> GCGCAGCCTGTACGGACATCA;> CCGTACA;> GGCTGC;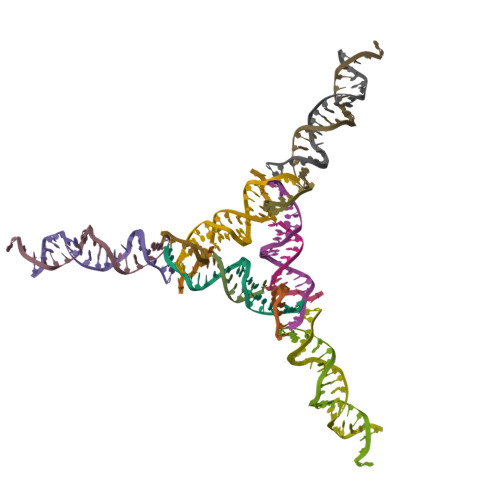> TCTGATGT;> GATGCTGACGTAGTAGCAGA;> GCTCTGCTACTACGTCAGCA> ELNRSQGIPFLEYKHFVTRTFFPKCSSLYEERYVLPSKTLNSQGGSPPQETHPLLGEWNIPEHCRPSMEEGISLFSSLLNNKHFLIVFVHALEQQKDFAVRDRCSLASLLTIALHGKLEYYTSIMKELLVDLIDASAAKNPKLMLRRTESVVEKMLTNWMSICMYGCLRETVGEPFFLLLCAIKQQINKGSIDAITGKARYTLNEEWLLRENIEAKPRNLNVSFQGCGMDSLSVRAMDTDTLTQVKEKILEAFCKNVPYSQWPRAEDVDLEWFASSTQSYVLRDLDDTSVVEDGRKKLNTLAHYKIPEGASLAMSLTDKKDSTLGRVKDLDTEKYFHLVLPTDELVEPKKSHRQSHRKKVLPEIYLTRLLSTKGTLQKFLDDLFKAILSIREDKPPLAVKYFFDFLEEQAEKRGISDPDTLHIWKTNSLPLRFWVNILKNPQFVFDIEKTDHIDACLSVIAQAFIDACSISDLQLGKDSPTNKLLYAKEIPEYRKTVQRYYKQIQDMTPLSEQEMNAHLAEESRKYQNEFNTNVAMAEIYKYAKRYRPQIMAALEANPTARRTQLQHKFEQVVALMENNIYECYSEA;> GPHMAALRPRLVFHTQLAHGSPTGRIEGFTNVKELYGKIAEAFRLPAAEVMFCTLNTHKVDMDKLLGGQIGLEDFIFAHVKGQRKEVEVFKSEE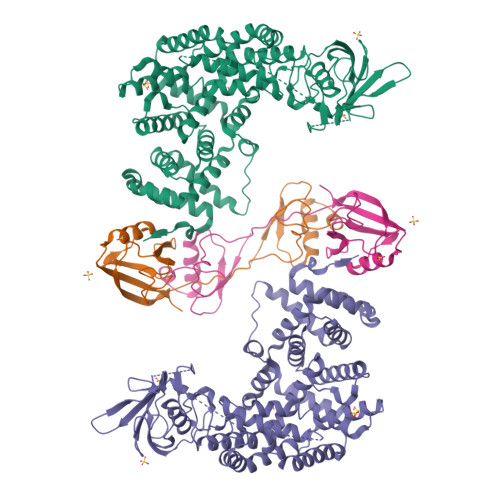ALGLTITDNGAGYAFIKRIKEGSVIDHIQLISVGDMIEAINGQSLLGCRHYEVARLLKELPRGRTFTLKLTEPRKAFDMISQRSAGGHPGSGPQLGTGRGTLRLRSRGPATVEDLPSAFEEKAIEKVDDLLESYMGIRDTELAATMVELGKDKRNPDELAEALDERLGDFAFPDEFVFDVWGAIGDAKVGRY> MGAEEEDTAILYPFTISGNDRNGNFTINFKGTP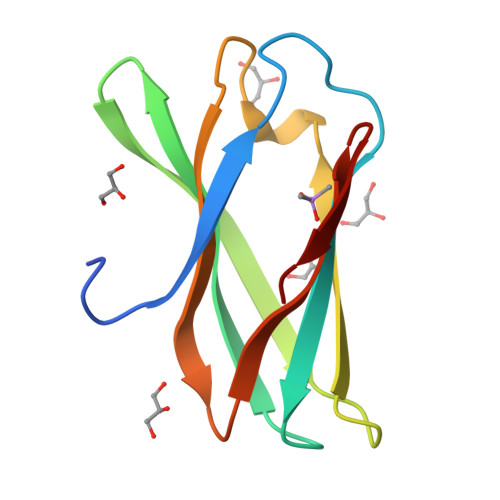NSTNNGCIGYSYNGDWEKIEWEGSCDGNGNLVVEVPMSKIPAGVTSGEIQIWWHSGDLKMTDYKALEHHHHHH> GAMGPVYKDLEIDVCNTPPPECINDLLKSVDSEEIREYCKKKKWIIPEI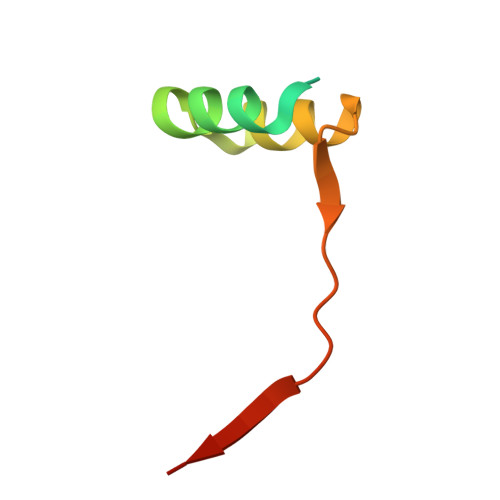PTNIERAMNQ>[2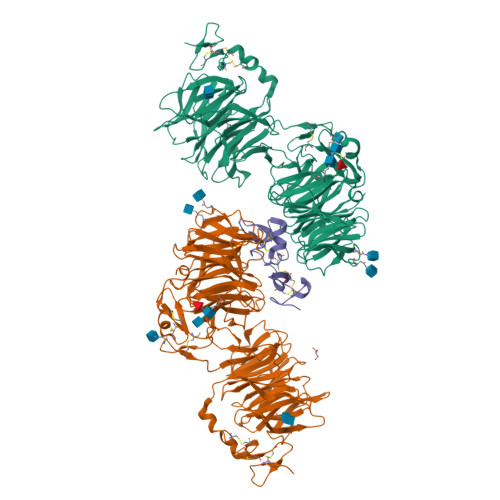x]ADPEAFLLFSRRADIRRISLETNNNNVAIPLTGVKEASALDFDVTDNRIYWTDISLKTISRAFMNGSALEHVVEFGLDYPEGMAVDWLGKNLYWADTGTNRIEVSKLDGQHRQVLVWKDLDSPRALALDPAEGFMYWTEWGGKPKIDRAAMDGSERTTLVPNVGRANGLTIDYAKRRLYWTDLDTNLIESSNMLGLNREVIADDLPHPFGLTQYQDYIYWTDWSRRSIERANKTSGQNRTIIQGHLDYVMDILVFHSSRQSGWNECASSNGHCSHLCLAVPVGGFVCGCPAHYSLNADNRTCSAPTTFLLFSQKSAINRMVIDEQQSPDIILPIHSLRNVRAIDYDPLDKQLYWIDSRQNMIRKAQEDGSQGFTVVVSSVPSQNLEIQPYDLSIDIYSRYIYWTCEATNVINVTRLDGRSVGVVLKGEQDRPRAIVVNPEKGYMYFTNLQERSPKIERAALDGTEREVLFFSGLSKPIALALDSRLGKLFWADSDLRRIESSDLSGANRIVLEDSNILQPVGLTVFENWLYWIDKQQQMIEKIDMTGREGRTKVQARIAQLSDIHAVKELNLQEYRQHPCAQDNGGCSHICLVKGDGTTRCSCPMHLVLLQDELSCGEPHHHHHHHHHH;> ADPMYHTKGQEGSVCLRSSDCASGLCCARHFWSKICKPVLKEGQVCTKHRRKGSHGLEIFQRCYCGEGLSCRIQKDHHQASNSSRLHTCQRHHHHHH> SGSDAAPGASKLRAVLEKLKLSRDDISTAAGMVKGVVDHLLLRLKCDSAFRGVGLLNTGSYYEHVKISAPNEFDVMFKLEVPRIQLEEYSNTRAYYFVKFKRNPKENPLSQFLEGEILSASKMLSKFRKIIKEEINDIKDTDVIMKRKRGGSPAVTLLISEKISVDITLALESKSSWPASTQEGLRIQNWLSAKVRKQLRLKPFYLVPKHAKEGNGFQEETWRLSFSHIEKEILNNH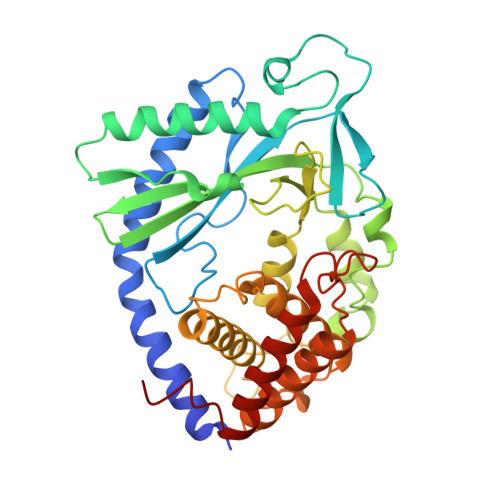GKSKTCCENKEEKCCRKDCLKLMKYLLEQLKERFKDKKHLDKFSSYHVKTAFFHVCTQNPQDSQWDRKDLGLCFDNCVTYFLQCLRTEKLENYFIPEFNLFSSNLIDKRSKEFLTKQIEYERNNEFPVFDEF>[2x]EVSQDLFNQFNLFAQYSAAAYCGKNNDAPAGTNITCTGNACPEVEKADATFLYSFEDSGVGDVTGFLALDNTNKLIVLSFRGSRSIENWIGNLNFDLKEINDICSGCRGHDGFTSSWRSVADTLRQKVEDAVREHPDYRVVFTGHALGGALATVAGADLRGNGYDIDVFSYGAPRVGNRAFAEFLTVQTGGTLYRITHTNDIVPRLPPREFGYS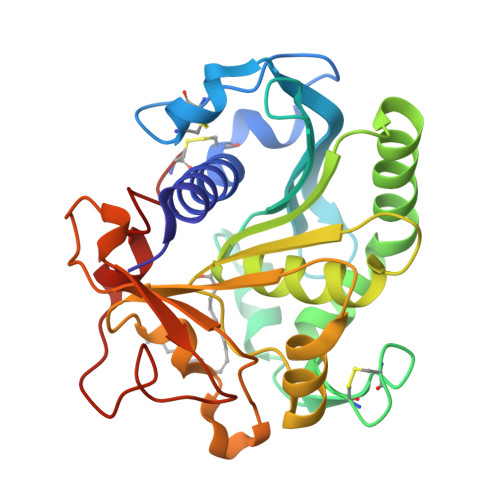HSSPEYWIKSGTLVPVTRNDIVKIEGIDATGGNNQPNIPDIPAHLWYFGLIGTCL> ST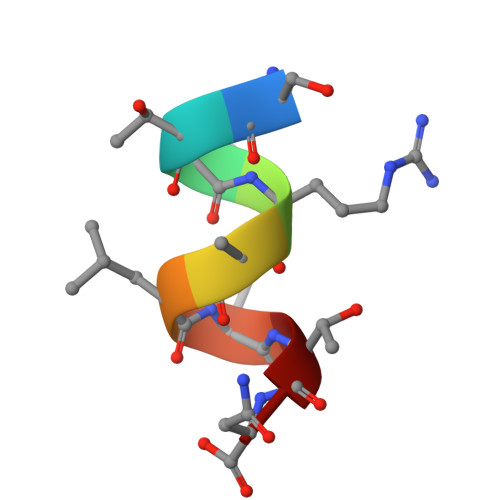LRALLTN>MLLEAIFHEAKGSYAYPISETQLRVRLRAKKGDVVRCEVLYADRYASPEEELAHALAGKAGSDERFDYFEALLECSTKRVKYVFLLTGPQGEAVYFGETGFSAERSKAGVFQYAYIHRSEVFTTPEWAKEAVIYQIFPERFANGDPSNDPPGTEQWAKDARPRHDSFYGGDLKGVIDRLPYLEELGVTALYFTPIFASPSHHKYDTADYLAIDPQFGDLPTFRRLVDEAHRRGIKIILDAVFNHAGDQFFAFRDVLQKGEQSRYKDWFFIED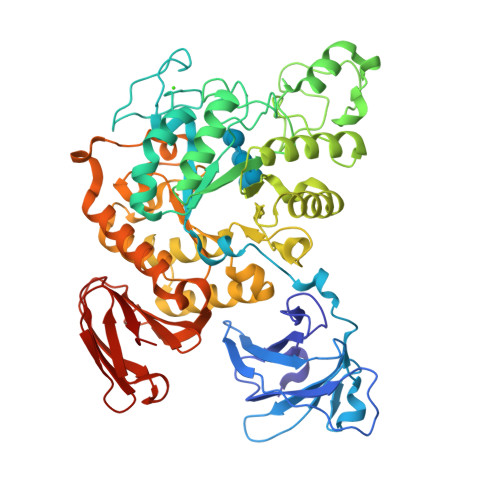FPVSKTSRTNYETFAVQVPAMPKLRTENPEVKEYLFDVARFWMEQGIDGWRLNVANEVDHAFWREFRRLVKSLNPDALIVGEIWHDASGWLMGDQFDSVMNYLFRESVIRFFATGEIHAERFDAELTRARMLYPEQAAQGLWNLLDSHNTERFLTSCGGNEAKFRLAVLFQMTYLGTPLIYYGDEIGMAGATDPDCRRPMIWEEKEQNRGLFEFYKELIRLRHRLASLTRGNVRSWHADKQANLYAFVRTVQDQHVGVVLNNRGEKQTVLLQVPESGGKTWLDCLTGEEVHGKQGQLKLTLRPYQGMILWNGR[2x]>TSEDACQDAEQPTRYETLFQALDRNGDGVVDIGELQEGLRNLGIPLGQDAEEKIFTTGDVNKDGKLDFEEFMKYLKDHEKKMKLAFKSLDKNNDGKIEASEIVQSLQTLGLTISEQQAELILQSIDVDGTMTVDWNEWRDYFLFNPVTDIEEIIRFWK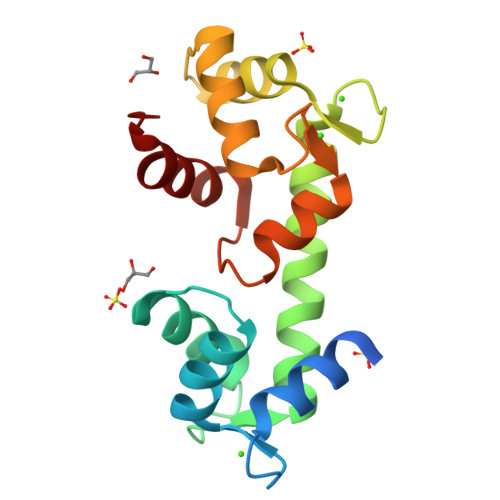HSTGIDI[3x]>[3x]MKKLTIGLIGNPNSGKTTLFNQLTGSRQRVGNWAGVTVERKEGQFSTTDHQVTLVDLPGTYSLTTISSQTSLDEQIACHYILSGDADLLINVVDASNLERNLYLTLQLLELGIPCIVALNMLDIAEKQNIRIEIDALSARLGCPVIPLVSTRGRGIEALKLAIDRYKAN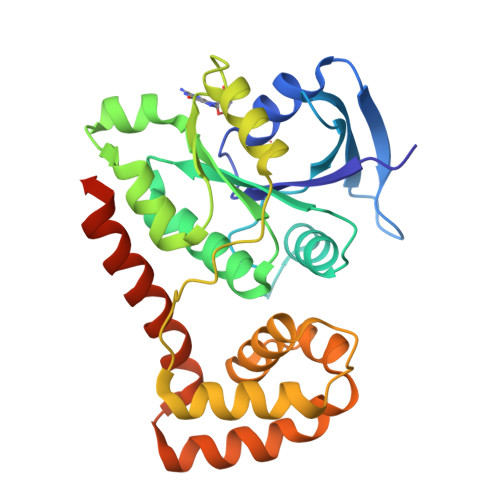ENVELVHYAQPLLNEADSLAKVMPSDIPLKQRRWLGLQMLEGDIYSRAYAGEASQHLDAALARLRNEMDDPALHIADARYQCIAAICDVVSNTLTAEPSRFTTAV>GASRPVVSGVASLGYEEQEVLKMAAAVEKT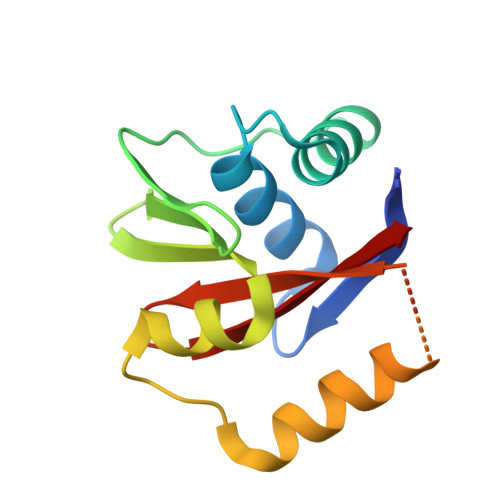ATHPIAKAIVNEAESLNLKTPETRGQLTEPGFGTLAEIDGRFVAVGSLEWVSDRFLKKNDSSDMVKLESLLDHKLSNTSSTSRYSKTVVYVGREGEGIIGAIAISD[2x]Canonical FGFs including FGF2 act as a paracrine and/or an autocrine by forming ternary complexes with FGF receptors (FGFRs) and heparan sulfate proteoglycans (HSPGs) on the cell surface. The FGFR-FGF-HSPG complex induces the dimerization of FGFR, resulting in a series of intracellular signaling cascades including the activation of MAPK/ERK pathway, PI3K/AKT pathway, and PLCγ pathway, etc. Through these signaling pathways, FGF2 regulates diverse cellular responses and has beneficial effects on wound healing, wrinkle reduction, and protection against neomycin-induced hair cell loss. While the therapeutic potentials of FGF2 are widely recognized, a significant challenge hindering its broader application is inherent instability.

Based on the calculation by in silico predictions, two FGF2 mutants with four-point mutations (FGF2-M1 with D28E/C78L/C96I/S137P and FGF2-M2 with D28E/C78I/C96I/S137P) were finally designed. We successfully solved the high-resolution (1.40 Å and 1.48 Å, respectively) crystal structures of FGF2-M1 and the FGF2-M2/SOS complex. On the other hand, SOS was used as an additive reagent to promote the crystallization of FGF2-M2 because it binds to the heparin-binding site of FGF2. In the crystal structure of the FGF2-M2/SOS complex, negatively charged SOS was bound to the positively charged HSPG-binding site harboring K128, R129, K134, and K138 through extensive electrostatic interactions. The RMSD value between the structures of the FGF2 mutants was 0.144 Å for all Cα atoms, indicating that the introduction of mutations did not affect the overall structure of FGF2. Both of them adopted the canonical β-trefoil fold, in which two sets of three β-hairpins are arranged with a pseudo-three-fold symmetry. The structures of FGF2-M1 and FGF2-M2 showed that leucine or isoleucine at position 78 were sandwiched by hydrophobic interactions consisting of P45, P58, H59, and L77. Thus, C78L and C78I seem to allow for better interactions with neighboring residues, which prefer a bit more hydrophobic and a bit larger amino acid; the hydropathy scales of leucine and isoleucine are 3.8 and 4.5, respectively, with their volumes of 166.7 Å3. The C96I mutation formed a van der Waals interaction with the methyl group of T98 at a distance ranging from 4.1 Å to 4.7 Å. The introduction of isoleucine at position 96 in the FGF2 mutants likely dictates the orientation of the T98 side-chain. Subsequently, the S137P mutation demonstrated an improvement in FGF2’s thermo-stability, as determined by SDS-PAGE and CD experiments. It was also identified through the crystal structures of FGF2-M1 and FGF2-M2; the substituted proline residue at position 137 forms CH-π interactions with W123 to stabilize the β10–β11 hairpin, a portion of the heparin-binding site of FGF2.

>[3x]MPALPEDGGSGAFPPGHFKEPKRLYCKNGGFFLRIHPDGRVDGVREKSDPHIKLQLQAEERGVVSIKGVIANRYLAMKEDGRLLASKIVTDECFFFERLESNNYNTYRSRKYTSWYVALKRTGQYKLGPKTGPGQKAILFLPMSAKS> GPLGSMEASCLELALEGERLCKSGDCRAGVSFFEAAVQVGTEDLKTLSAIYSQLGNAYFYLHDYAKALEYHHHDLTLARTIGDQLGEAKASGNLGNTL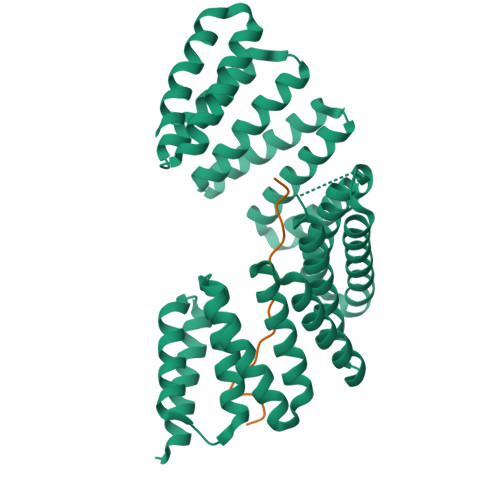KVLGNFDEAIVCCQRHLDISRELNDKVGEARALYNLGNVYHAKGKSFGCPGPQDVGEFPEEVRDALQAAVDFYEENLSLVTALGDRAAQGRAFGNLGNTHYLLGNFRDAVIAHEQRLLIAKEFGDKAAERRAYSNLGNAYIFLGEFETASEYYKKTLLLARQLKDRAVEAQSCYSLGNTYTLLQDYEKAIDYHLKHLAIAQELNDRIGEGRACWSLGNAYTALGNHDQAMHFAEKHLEISREVGDKSGELTARLNLSDLQMVLGLSYSTNNSIMSENTEIDSSLNGVRPKLGRRHSMENMELMKLTPEK;> GPGSDLPPKVVPSKQLLHSDHMEMEPETMETKSVTDYFSKLHMGSVAYSCTSEFHHHHHH> QEEWETV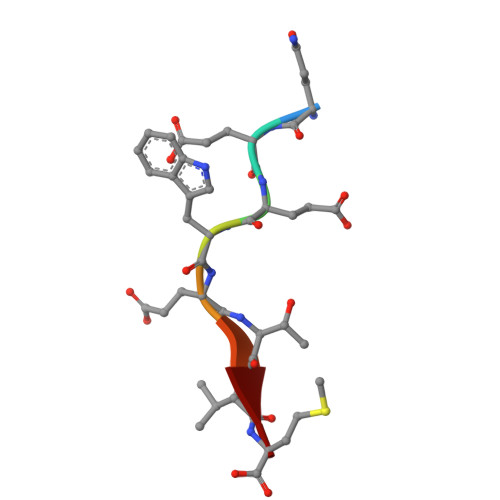M> KAQKKNRNKLRRQ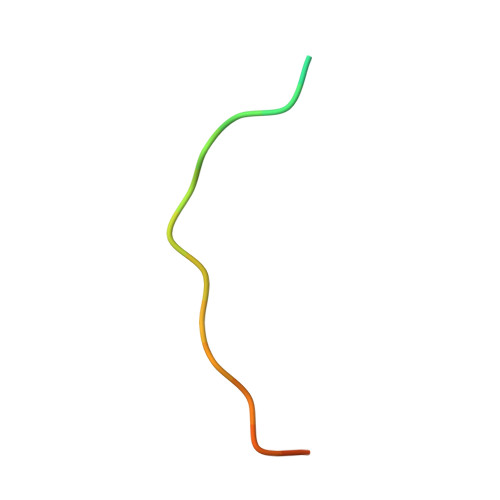HDYDTFVDL> MARALRDISLFNDIRKDQNSAGAKHERYNMRDLRSKKNQHVNGIDDYEDDSLDRFIRRKKSRVVKYIPSLSAYNVFNEFPYYPTSASQLLDGKLDEFLMLSEQYKSRLPKIRKLGWNRFKPIGINKTMYELEMLRSRARAQNAEGNNEEDFRQHDSREEDPRNNGSIGRVILPHILQENEEYDTGEGVTGLHSMPNDSMAILANNSANNSQNEEVSEEDEISYDYDAEFDHVVDEDDNEEGEVPGEGVEGIEVQRERIVPDDLLMRPTSLSRSLQQFVEEAHHLDRNPYDIDSDNDGEDSKVELDMNPD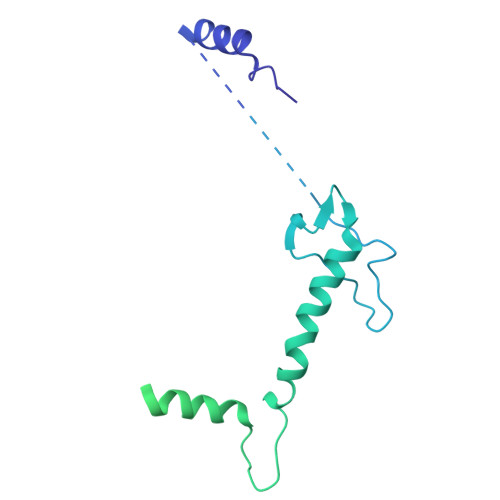FEDDVGREHDYNSEYSQEPTSYGGITPDLASNWRNWTRERITSLDELMERRARQQRGQD>SNAMEIIPIPADSYTLGFIGAGKMAESIAKGAVRSGVLSPSRIKTAIHSNPARRTAFESIGITVLSSNDDVVRDSNVVVFSVKPQLLKDVVLKLKPLLTKDKLLVSVAAGIKMKDLQEWAGHERFIRVMPNTAATVGEAASVMSLGGAATEEDANLISQLFGSIGKIWKADDKYFDAITGL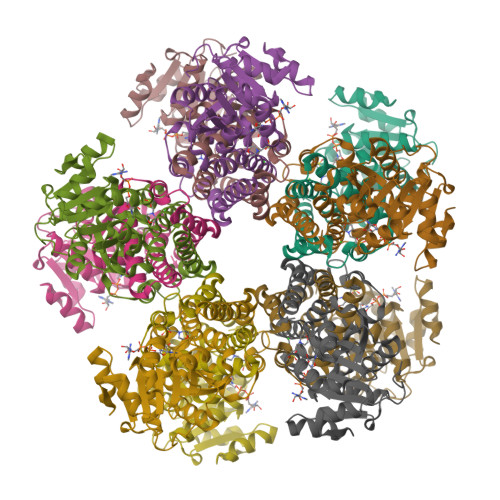SGSGPAYIYLAIEALADGGVAAGLPRDLALSLASQTVLGAASMATQSGKHPGQLKDDVTSPGGTTIAGVHELEKAGFRGILMNAVVAAAKRSQELS[10x]> MSRKRNRNRSVQVAKATSEQLNVSRMRMSEQGTFALAKVQVDSERMKAEEIRWPHLIGTAESMKQDATVATGLDMLYTFVEKAFKDFKVIPGESEESKKAAKFIEYCLKNMEGQTLRQFARDAATFNEYGLSVVEKVYTQIAVGEYVGKYKVKNLAFRPQASLSRTNPIVYNSDGSAIVGIKQSLSAFQNYTASEIGVGGVSTRMSDVIIPISRVMLMNTGGSSSQALGVSPLVGCYRAWREKILIENLEVVGATKDMGGVIELKIPSQILNKAAMDPSSPEADMVRGLMSDAANAHSGEQSFFMLPSDTKDNAPQYSMTLKGIDGMGKQYSTAQLISDRKKSILDRLGAGFINVGNDK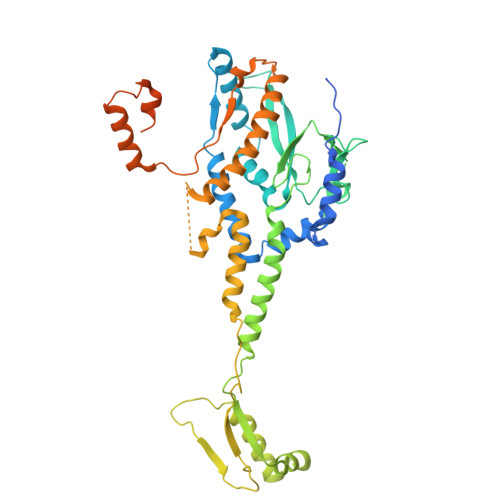GGSYNLSESKQTIHTQFVQRVNEIILEALNENLLPQLLALNDIRLPETEMPYVKAGEIVDVDMEGFSKAIQRIGAVGYLPKTPKVINRVLEVLGIDEKIEEDISQEELMKLLGEDTSRAGDGMTKGSSGNGTGKISASRDNSAANLDN> AARYDDVLYFPASRYPETGAHISDAIKAGHADVCTIERSGADKRRQESLKGIPTKPGFDRDEWPMAMCEEGGKGASVRYVSSSDNRGAGSWVGNRLNGYADGTRIL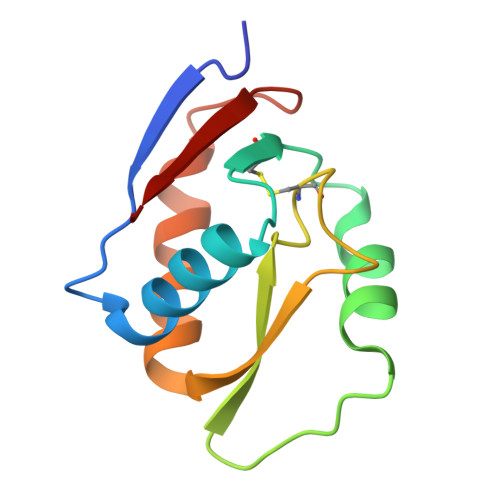FIVQ>[2x]MVVIGEKFPEVEVKTTHGVIKLPDYF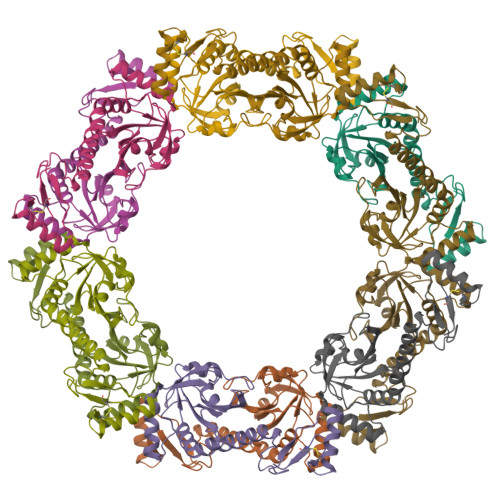AEQGKWFVLFSHPADFTPVCTTEFYAMQKRVDQFRELGVEPIGLSVDQVFSHIKWMEWIKENLGEEITFPVIADDRGELADKLGMIPSGATITARAVFIVDDKGIIRAIVYYPAEVGRDWDEILRLVKALKVSDEKGVALPHKWPNNELIGDKAIVPPASTVDEVKQREEAKAKGEIECYDWWFCYKKLE>GDPAPLEQMRLTEQALEQAKAVGATDDVAELKLAQDKYAAAQIAMTAESYKKARLLAEQAELDARLAESKVLTQKSKDQLGELDKSLK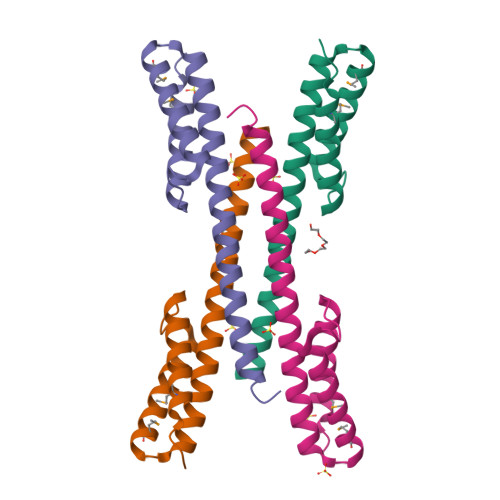RLRKQLGETD[4x]>[2x]ASLTEIEHLVQSVCKSYRETCQLRLEDLLRQRSNIFSREE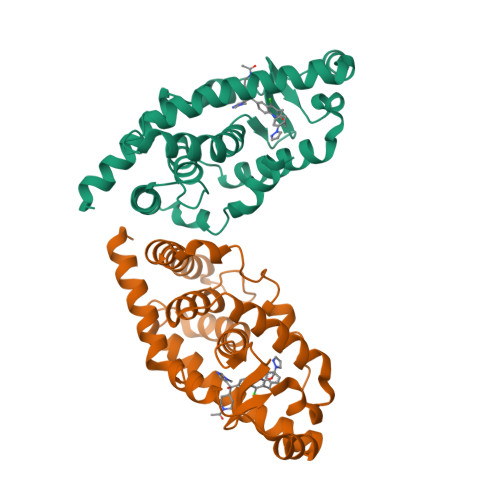VTGYQRKSMWEMWERCAHHLTEAIQYVVEFAKRLSGFMELCQNDQIVLLKAGAMEVVLVRMCRAYNADNRTVFFEGKYGGMELFRALGCSELISSIFDFSHSLSALHFSEDEIALYTALVLINAHRPGLQEKRKVEQLQYNLELAFHHHLCKTHRQSILAKLPPKGKLRSLCSQHVE> MVVIGEKFPEVEVKTTHGVIKLPDYFAEQGKWFVLFSHPADCTPVSTTEFYAMQKRVDQFRELGVEPIGLSVDQVFSHIKWMEWI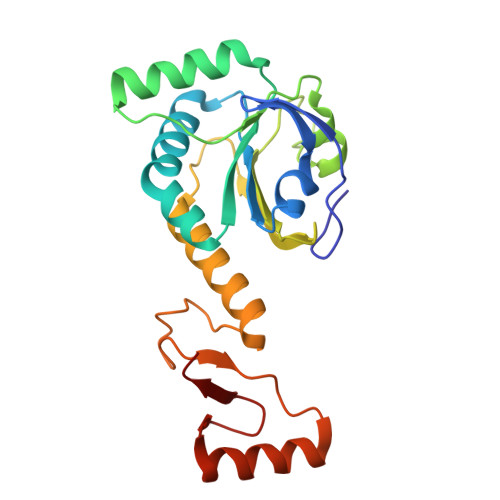KENLGEEITFPVIADDRGELADKLGMIPSGATITARAVFIVDDKGIIRAIVYYPAEVGRDWDEILRLVKALKVSDEKGVALPHKWPNNELIGDKAIVPPASTVDEVKQREEAKAKGEIESYDWWFSYKKLE> GPMTTTERPDLAWLDEVTMTQLERNPYEVYERLRAEAPLAFVPVLGSYVASTAEVCREVATSPDFEAVITPAGGRTFGHPAIIGVNGDIHADLRSMVEPALQPAEVDRWIDDLVRPIARRYLERFENDGHAELVAQYCEPVSVRSLGDLLGLQEVDSDKLREWFAKLNRSITNAAVDENGEFANPEGFAEGDQAKAEIRAVVDPLID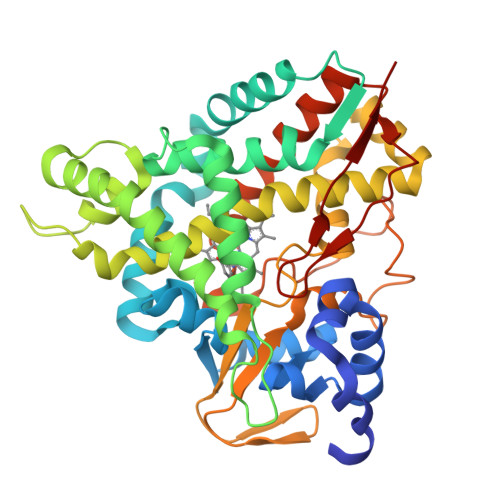KWIEHPDDSAISHWLHDGMPPGQTRDREYIYPTIYVYLLGAMQEPGHGMASTLVGLFSRPEQLEEVVDDPTLIPRAIAEGLRWTSPIWSATARISTKPVTIAGVDLPAGTPVMLSYGSANHDTGKYEAPSQYDLHRPPLPHLAFGAGNHACAGIYFANHVMRIALEELFEAIPNLERDTREGVEFWGWGFRGPTSLHVTWEV> MSLPHVILTVLSTRDATGYDITKEFSASIGYFWKASHQQVYRELNKMGEQGLV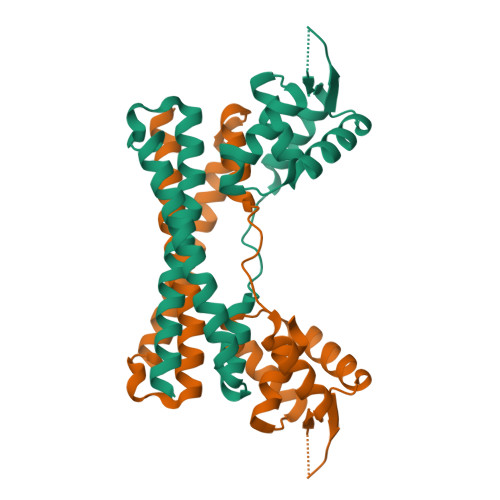TCVLEPQEGKPDRKVYSITQAGRSALGEWFDQPTAHPTVRDEFSAKLMACSVQSAEPYRLQLAELVEESRKLVAHYQEIEAAYYANPAVLDKQQRLERLTLRRNLLVRQAWIQWADEVLAELNAMA> MANTPEHIGNDLKLFKDSSCTSLKPDVKNTSAFQSDAMKELATKILAGHYKPDYLYAEYRALPSPRQTGKNLRIGDGFSKYDNMTGVYLEKGRHVVLVGKTEGQEISLL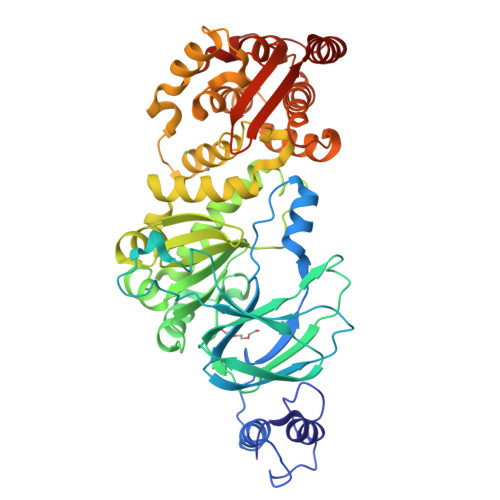LPNLMRKPAEGVQPTKDPNGWGLHKKQIPLKEGINIIDVETPANAYISYFTEDAGKAPKIPVHFVTGKANGYFDTTRGDTNKDWVRLLDQAVSPIMDARGKYIQVAYPVEFLKKFTKDRGTELINAYDKLIGIQYQLMGLDKYGKIPENRVLARVNFNYYMFRDGDGVAYLGNDGTMRMVTDPENVLKGDACWGFSHEVGHVMQMRPMTWGGMTEVSNNIFSLQAAAKTGNESRLKRQGSYDKARKEIIEGEIAYLQSKDVFNKLVPLWQLHLYFTKNGHPDFYPDVMEYLRNNAGNYGGNDTVKYQFEFVKACCDVTKTDLTDFFEKWGFFKPGKFHIGDYAQYDFNVTPEMVEETKKWIAGKGYPKPETDITELSE>ETGPHMFWTGWGPWERCTAQCGGGIQARRRICENGPDCAGCNVEYQSCNTNPCPELKKTTPWTPWTPVNISDNGGHYEQRFRYTCKARLADPNLLEVGRQRIEMRYCSSDGTSGCSTGTLEVLFQ[2x]

Semaphorin-5A (Sema5A) is a bifunctional guidance cue exerting attractive and inhibitory effects on neuronal growth through the interaction with heparan sulfate (HS) and chondroitin sulfate (CS) glycosaminoglycans (GAGs), respectively. TSRs are a unique feature of Sema5s and enable interactions with heparan sulfate (HS) and chondroitin sulfate (CS) glycosaminoglycan (GAG) chains linked to the protein core of proteoglycans. We determined four Sema5ATSR3-4 crystal structures to high resolution (1.56–2.72 Å); apo state and complexes with nitrate, sulfate, and the heparin disaccharide mimetic sucrose octasulfate (SOS). Sema5ATSR3-4 is a rod-like dimer; superposition of the various structures indicates TSR3-TSR4 inter-domain angle differences, which may contribute conformational flexibility to the Sema5A ectodomain.

The novel architecture of TSR4 supports two symmetrically positioned ~20 × 20 Å-sized shallow cavities on the opposing sides of the Sema5A dimer. Positively charged and polar residues (K505, T732, K734, R747, R749) from both monomers contribute to each of these sites, together providing a notable positive electrostatic surface potential. There is an absence of clear electron density for key Sema5A GAG site sidechains, R747’ and R749’ in the apo Sema5ATSR3-4 structure. The conformational flexibility of these residues is consistent with an adaptable binding site that can accommodate GAG binding partners in vivo.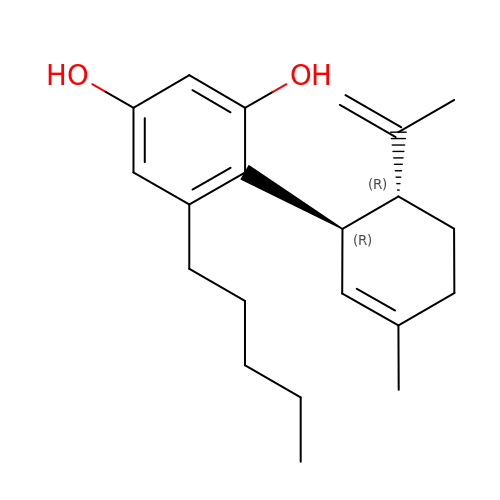(1'R,2'R)-5'-methyl-6-pentyl-2'-(prop-1-en-2-yl)-1',2',3',4'-tetrahydro[1,1'-biphenyl]-2,4-diol | C21 H30 O2 | YWEZXUNAYVCODW-RBUKOAKNSA-N>[2x]MGSSHHHHHHSSGLVPRGSNQPQTTSVLIRKYAIGDYSKLLEGATLQLTGDNVNSFQARVFSSNDIGERIELSDGTYTLTELNSPAGYSIAEPITFKVEAGKVYTIIDGKQIENPNKEIVEPYSVEAYNDFEEFSVLTTQNYAKFYYAKNKNGSSQVVYCFNADLKSPPDSEDGGKTMTPDFTTGEVKYTHIAGRDLFKYTVKPRDT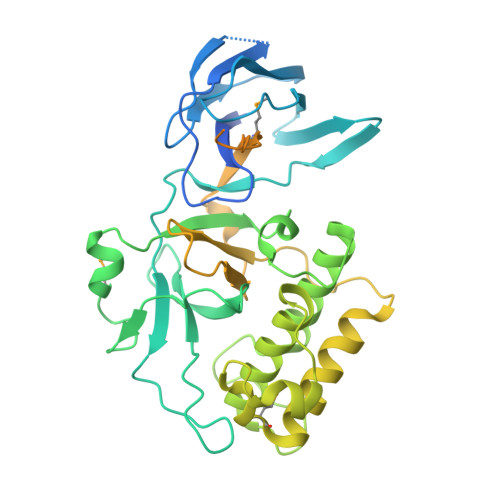DPDTFLKHIKKVIEKGYREKGQAIEYSGLTETQLRAATQLAIYYFTDSAELDKDKLKDYHGFGDMNDSTLAVAKILVEYAQDSNPPQLTDLDFFIPNNNKYQSLIGTQWHPEDLVDIIRMEDKKEVIPVTHNLTLRKTVTGLAGDRTKDFHFEIELKNNKQELLSQTVKTDKTNLEFKDGKATINLKHGESLTLQGLPEGYSYLVKETDSEGYKVKVNSQEVANATVSKTGITSDETLAFENNKEPVVPT>[2x]SLLNVPAGKDLPEDIYVVIEIPANADPIKYEIDKESGALFVDRFMSTAMFYPCNYGYINHTLSLNGDPVDVLVPTP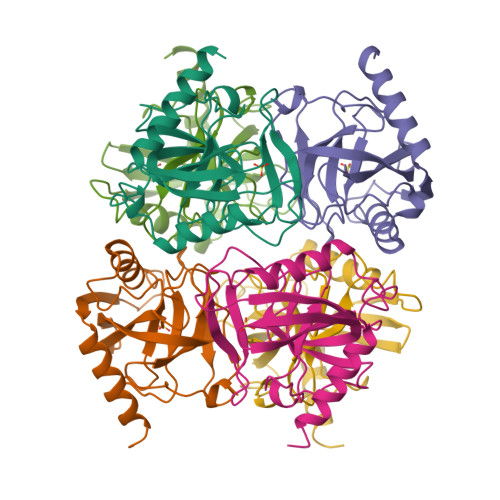YPLQPGSVIRCRPVGVLKMTDEAGEDAKLVAVPHSKLSKEYDHIKDVNDLPELLKAQIAHFFEHYKDLEKGKWVKVEGWENAEAAKAEIVASFERAKNK> MDLSELERDNTGRCRLSSPVPAVCLKEPCVLGVDEAGRGPVLGPMVYAICYCPLSRLADLEALKVADSKTLTENERERLFAKMEEDGDFVGWALDVLSPNLISTSMLGRVKYNLNSLSHDTAAGLIQYALDQNVNVTQVFVDTVGMPETYQARLQQHFPGIEVTVKAKADSLFPVVSAASIFAKVARDKAVKNWQFVENLQDLDSDYGSGYPNDPKTKAWLRKHVDPVFGFPQFVRFSWSTAQAILEKEAEDVIWEDSEAEEDPERPGKITSYFSQGPQTCRPQAPHRYFQERG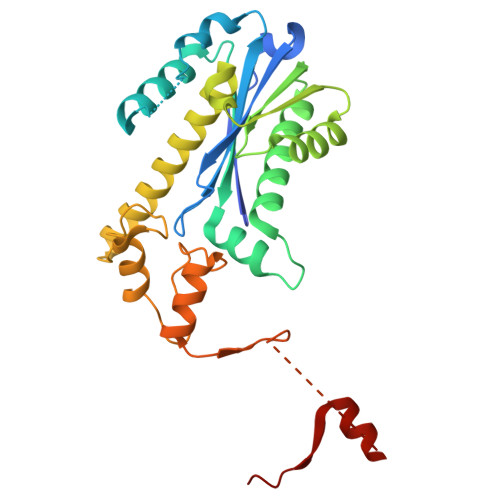LEAASSL>MSTLYSTQVKAVGGRSGTIRSEDGILELKLALPKELGGKGDATNPEQLFAAGYAACFGNAVIHVTRSNKEYKIR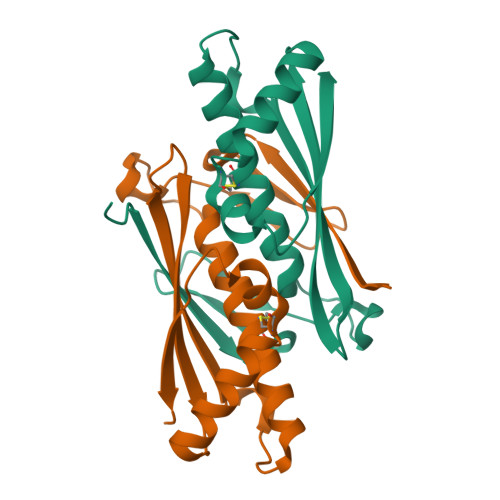DNDVEVLSTVGIVANGNGGFALTVHLDVTLSGISQADAEKIVEQTHQVCPYSNAIRGNIQVSTTVYTK[4x]(1S,2S,3S,4S,5R,6R)-5-amino-6-(hydroxymethyl)cyclohexane-1,2,3,4-tetrol | C7 H15 N O5 | 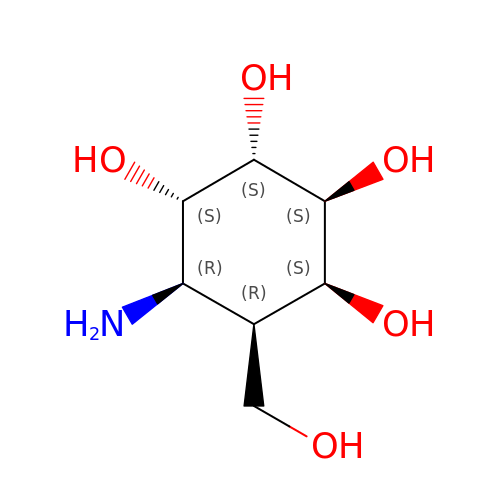SWVTZDDSAFUTKS-OUIVRQFQSA-N> AAPEVLADFHGEMGGCDSCHVSDKGGVTNDNLTHENGQCVSCHGDLKELAAAAPKDKVSPHKSHLIGEIACTSCHKGHEKSVAYCDACHSFGFDMPFGGKWERKFVPVDADKAAQDKAIAAGVKETTDVVIIGSGGAGLAAAVSARDAGAKVILLEKEPIPGGNTKLAAGGMNAAETKPQAKLGIEDKKQIMIDDTMKGGRNINDPELVKVLANNSSDSIDWLTSMGADMTDVGRMGGASVNRSHRPTGGAGVGAHVAQVLWDNAVKRGTDIRLNSRVVRILEDASGKVTGVLVKGEYTGYYVIKADAVVIAAGGFAKNNERVSKYDPKLKGFKATNHPGATGDGLDVALQAGAATRDLQYIQAHPTYSPAGGVMITEAVRGNGAIVVNREGNRFMNEITTRDKASAAILQQKGESAYLVFDDSIRKSLKAIEGYVHLNIVKEGKTIEELAKQIDVPAAELAKTVTAYNGFVKSGKDAQFERPDLPRELVVAPFYALEIAPAVHHTMGGLVIDTK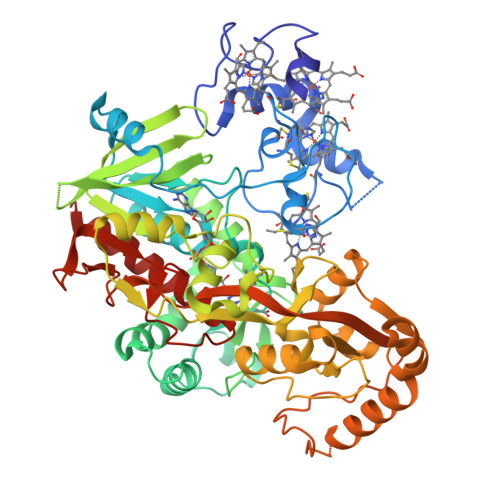AEVKSEKTAKPITGLYAAGEVTGGVHGANRLGGNAISDIVTYGRIAGASAAKFAKDN> SNAMKIGIIGAGQLARMLSLAGTPLGLEFHCLGKNGDCAEEVVKTVTDIELTKVNDVVAWAKQFDVITFENENISHELIKAINHEVSVYPSAKAIAISQDRLLEKSFMQDHGIATAKFVNIDSLAKLQSAVDDHGLPAILKTRRFGYDGKGQFVIRSQEDITKAWDVLKDAPDGLIYEAFVDFDYEVSQICTADLKGNIAFYPLARNTHKQGIIVESEAPFENVVLAEKAQQIAKILVKEFAYVGTLAIEFFVKGDELIVN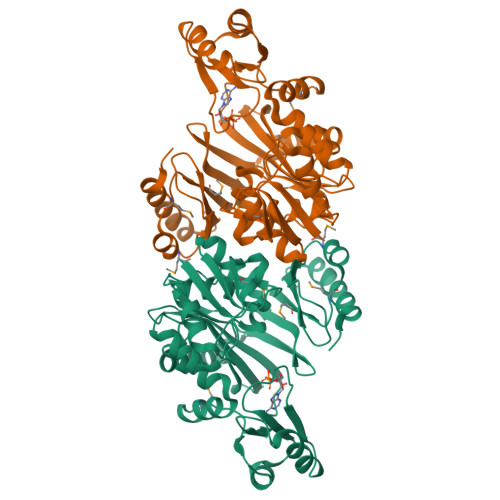EIAPRVHNSGHWSIDGAVTSQFENHVRAIAGLILGDTTSRKTVMLNCIGGMPATKDLAALDRVKIHSYNKEPRKGRKVGHLNLNLNDETDEYQLLQVKKLIALSEEI> ANPLYQKHIISINDLSRDDLNLVLATAAKLKANPQPELLKHKVIASCFFEASTRTRLSFETSMHRLGASVVGFSDSANTSLGKKGETLADTISVISTYVDAIVMRHPQEGAARLATEFSGNVPVLNAGDGSNQHPTQTLLDLFTIQETQGRLDNLHVAMVGDLKFGRTVHSLTQALAKFDGNRFYFIAPDALAMPQYILDMLDEKGIAWSLHSSIEEVMAEVDILYMTRVQKERLDPSEYANVKAQFVLRASDLHNAKANMKVLHPLPRVDEIATDVDKTPHAWYFQQAGNGIFARQALLALVLNRDLVL;>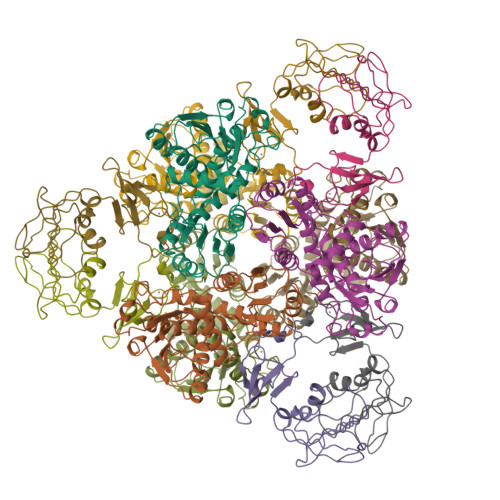 QVEAIKRGTVIDHIPAQIGFKLLSLFKLTETDQRITIGLNLPSGEMGRKDLIKIENTFLSEDQVDQLALYAPQATVNRIDNYEVVGKSRPSLPERIDNVLVCPNSNCISHAEPVSSSFAVRKRANDIALKCKYCEKEFSHNVVLAN>GGSKKHTGYVGLKNQGATCYMNSLLQTLFFTNQLRKAVYMMPTEGDDSSKSVPLALQRVFYELQHSDKPVGTKKLTKSFGWETLDSFMQHDVQELCRVLLDNVENKMKGTCVEGTIPKLFRGKMVSYIQCKEVDYRSDRREDYYDIQLSIKGKKNIFESFVDYVAVEQLDGDNKYDAGEHGLQEAEKGVKFLTLPPVLHLQLMRFMYDPQTDQNIKINDRFEFPEQLPLDEFLQKTDPKDPANYILHAVLVHSGDNHGGHYVVYLNPKGDGKWCKFDDDVVSRCTKEEAIEHNYGGHDDDLSVRHCTNAYMLVYIRESKLSEVLQAVTDHDIPQQLVERLQEEKRIEAQKRKERQE[2x]

In recent years, the cysteine protease ubiquitin‐specific protease 7 (USP7), also known as herpes‐associated ubiquitin‐specific protease (HAUSP), has become one of the most extensively studied deubiquitinases. This is mainly due to its role in tumorigenesis‐associated signaling pathways and its interaction with the tumor suppressor p53 and the oncogenic ubiquitin E3 ligase murine double minute (MDM2). Herein, after a design based on molecular docking experiments, we report the synthesis of a series of mildly electrophilic compounds that covalently modify the catalytic cysteine 223 in USP7 through a nucleophilic aromatic substitution (SNAr) reaction.

Finally, a co‐crystal structure revealed that the prototype compound (7a) arylates the catalytic cysteine in the apo form of USP7 via an unconventional binding mode near the catalytic triad. The electron density of the new bond at Cys223 is clearly visible, whereas no additional density at any other cysteines or amino acids could be observed. As expected, the compound reacted in an SNAr reaction with the fluorine atom being displaced. The structure confirmed that the catalytic cysteine is modified in the inactive state of USP7, where it is less nucleophilic due to the disassembly of the catalytic triad. Compound 7a generally shows an unconventional binding mode compared with all crystal structures, currently published in the PDB. It reaches deep into the region where the catalytic triad amino acids His464 and Asp481 are located. Other published compounds are all oriented in the other direction of the ubiquitin binding channel. However, the exact binding mode must be interpreted with caution as compound 7a is close to crystal contacts. The omit map of compound 7a is shown in Figure 11A,B. The binding mode determined experimentally is closer to the ubiquitin site than the docking pose, with less extension into the pocket near the catalytic aspartate and histidine.2-[[3-[(2E)-2-[1,3-bis(oxidanylidene)-1-phenyl-butan-2-ylidene]hydrazinyl]phenyl]sulfonylamino]benzoic 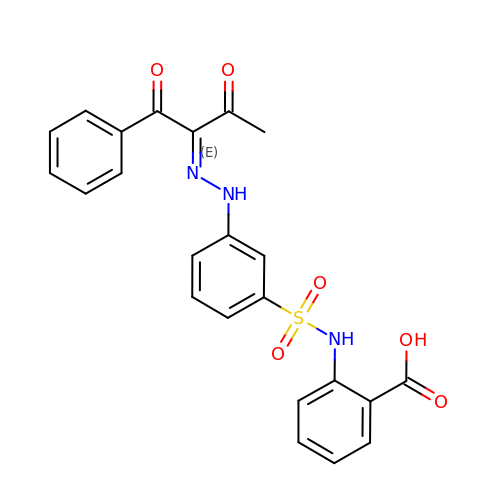acid | C23 H19 N3 O6 S | SOWABNTWBBBOPH-NJNXFGOHSA-N>[4x]PHMQPFDSGHDDLVHDVVYDFYGRHVATCSSDQHIKVFKLDKDTSNWELSDSWRAHDSSIVAIDWASPEYGRIIASASYDKTVKLWEEDPDQEECSGRRWNKLCTLNDSKGSLYSVKFAPAHLGLKLACLGNDGILRLYDALEPSDLRSWTLTSEMKVLSIPPANHLQSDFCLSWCPSRFSPEKLAVSALEQAIIYQRGKDGKLHVAAKLPGHKSLIRSISWAPSIGRWYQLIATGCKDGRIRIFKITEKLSPLASEESLTNSNMFDNSADVDMDAQGRSDSNTEEKAELQSNLQVELLSEHDDHNGEVWSVSWNLTGTILSSAGDDGKVRLWKATYSNEFKCMSVITAQQ;>MTIDDSNRLLMDVDQFDFLDDGTAQLSNNKTDEEEQLYKRDPVSGAILVPMTVNDQPIEKNGDKMPLKFKLGPLSYQNMAFITAKDKYKLYPVRIPRLDTSKEFSAYVSGLFEIYRDLGDDRVFNVPTIGVVNSNFAKEHN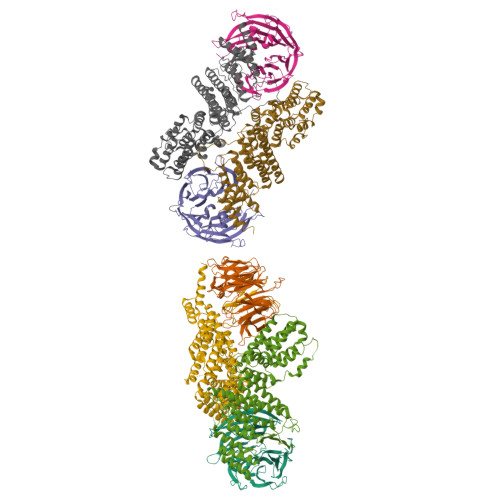ATVNLAMEAILNELEVFIGRVKDQDGRVNRFYELEESLTVLNCLRTMYFILDGQDVEENRSEFIESLLNWINRSDGEPDEEYIEQVFSVKDSTAGKKVFETQYFWKLLNQLVLRGLLSQAIGCIERSDLLPYLSDTCAVSFDAVSDSIELLKQYPKDSSSTFREWKNLVLKLSQAFGSSATDISGELRDYIEDFLLVIGGNQRKILQYSRTWYESFCGFLLYYIPSLELSAEYLQMSLEANVVDITNDWEQPCVDIISGKIHSILPVMESLDSCTAAFTAMICEAKGLIENIFEGEKNSDDYSNEDNEMLEDLFSYRNGMASYMLNSFAFELCSLGDKELWPVAIGLIALSATGTRSAKKMVIAELLPHYPFVTNDDIEWMLSICVEWRLPEIAKEIYTTLGNQMLSAHNIIESIANFSRAGKYELVKS[4x]>MTMAGGRRGLVAPQNTFLENIVRRSNDTNFVLGNAQIVDWPIVYSNDGFCKLSGYHRAEVMQKSSTCSFMYGELTDKDTIEKVRQTFENYEMNSFEILMYKKNRTPVWFFVKIAPIRNEQDKVVLFLCT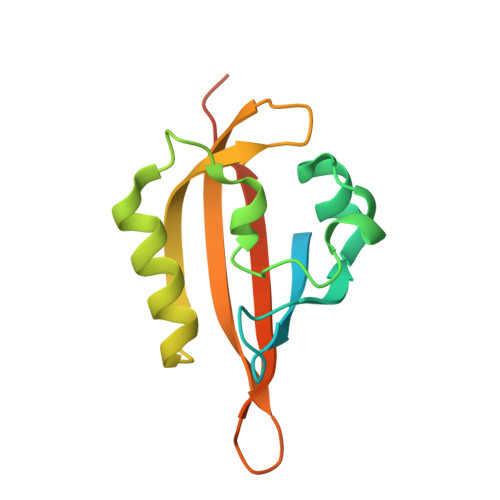FSDITAFKQPIEDDSCK[6x]>[2x]RETHFLKIPIGDLNIITQDNMKSCQMTTPVIDVIQMLTQGRVSSVPIIDENGYLINVYEAYDVLGLIKGGIYNDLSLSVGEALMRRSDDFEGVYTCTKNDKLSTIM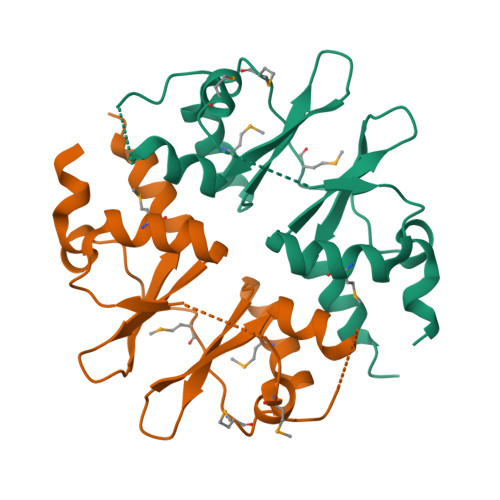DNIRKARVHRFFVVDDVGRLVGVLTLSDILKYILLGSN Although amyloid fibers and oligomers of two proteins, tau and amyloid-β, have been identified in association with this disease, the development of diagnostics and therapeutics has proceeded to date in a near vacuum of information about their structures. Here we report the first atomic structures of small molecules bound to amyloid. These are of the dye orange-G, the natural compound curcumin, and the Alzheimer's diagnostic compound DDNP bound to amyloid-like segments of tau and amyloid-β. Negatively charged orange-G wedges into a specific binding site between two sheets of the fiber, combining apolar binding with electrostatic interactions, whereas uncharged compounds slide along the cavity. The amyloid components in our structures are steric zippers formed by stacks of six-residue segments from Alzheimer-related proteins.

The KLVFFA segment (residues 16–21) from Aβ contains apolar residues that participate in a hydrophobic spine in Aβ fibers and itself acts as an inhibitor of Aβ fibrillation. We previously determined the atomic structure of the KLVFFA segment in three crystal forms; all show the common steric zipper motif associated with amyloid fibers (Colletier et al. unpublished results). The co-crystallization of KLVFFA with orange-G resulted in deeply colored crystals. Mass spectrometric analyses of the crystals showed high abundance of orange-G (∼1∶1 molar stoichiometry with KLVFFA). Determination of the structure revealed a novel, fourth form of the KLVFFA steric zipper, with orange-G wedged between the paired β-sheets of the zipper, leading to partial opening of the zipper. Stabilization of the binding arises from packing of the aromatic rings of orange-G against the apolar, partially aromatic spine of KLVFFA. At the interface between orange-G and KLVFFA, a total of 500 Å2 of apolar surface area is covered, corresponding very roughly to a binding energy of 9 kcal/mol, or a dissociation constant of ∼0.3 µM. Further stabilization arises from the salt links between the negatively charged sulfonic acid groups of orange-G and positively charged lysine side chains from both β-sheets. The differences in the binding cavities between the KLVFFA and VQIVYK fibers may account for the higher molecular stoichiometry within the KLVFFA-orange-G crystals observed by mass spectrometric analyses, and the correspondingly greater order of this complex.

>[4x]KLVFFA>MGSSHHHHHHHSSGLVPRGSHMDPVSVWGNTPLATVDPEIHDLIEKEKRRQCRGIELIASENFTSFAVIEALGSALTNKYSEGMPGNRYYGGNEYIDQIENLCRSRALQAFHLDAQSWGVNVQPYSGSPANFAAYTAVLNPHDRIMGLDLPSGGHLTHGYYTSGGKKISATSIYFESLPYKVNSTTGYIDYDRLEEKALDFRPKLIICGGSAYPRDWDYKRFREVADKCGALLLCDMAHTSGLVAAQEVNSPFEYCDIVTTTTHKSLRGPRAGMIFYRKGPKPPKKGQPENAVYDFEDKINFAVFPSLQGGPHNHQIGALAVALKQAASPGFKAYAKQVKANAVALGKYLMGKGYSLVTGGTENHLVLWDLRPLGLTGYKVEKLCDLCNITVNKNAVFGDSSALAPGGVRIGAPAMTSRGLVEKDFEQIGEFLHRAVTLTLEIQKEHGKLLKDFNKGLVNNKAIEDL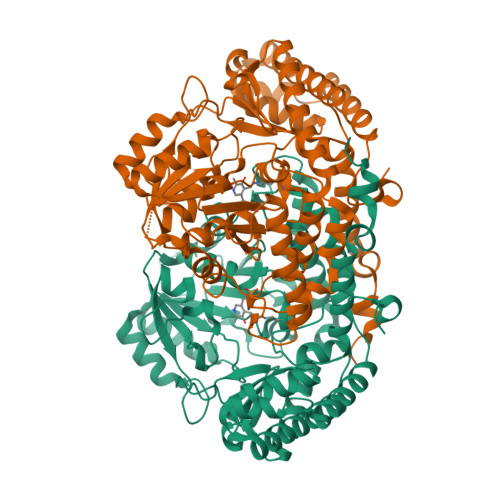KADVEKFSALFDMPGFLVSEMKYKD[2x]>GSSQAKPP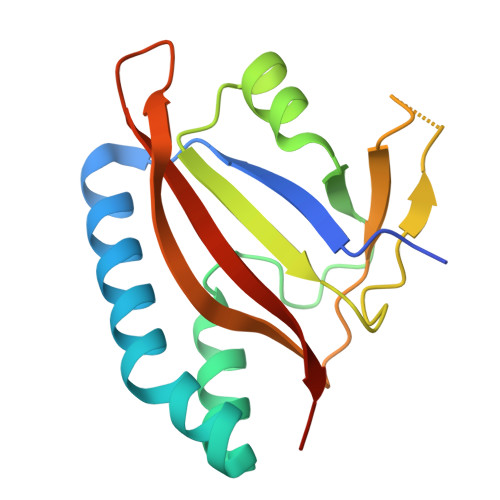TRLFRGLNLSEEFTKGLIDQANAMIANTTERLFTDHSPEAFKQIKLNDLSKMSGRTNASTTTEIKLVKETWDSNVIFEMLDPDGLLHSKQVGRHGEGTESEFSVYLPEDVALVPVKVTLDGKTQKGENRYVFTFVAVKSPDFTP[4x]> MFTRFVTQPTLLTQTQRALFSALTKKQKMEVTLRTPYKEYLANFDGFSRITAKTNEASLVIQNKTPASLYVLPPGPLKIRFTSEVKNVSGDFLHTGGWVIVHADNTCEI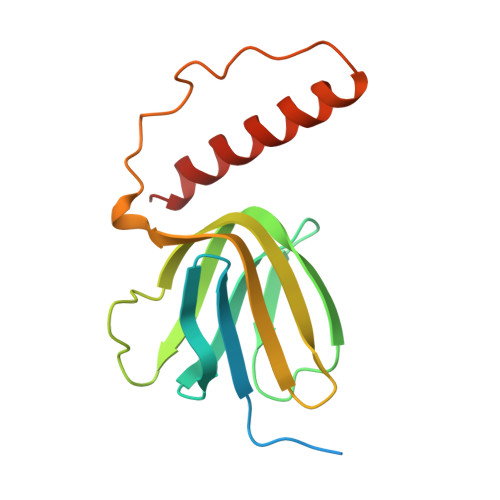NVMDLFDRKEVRADQFEKGNIQDLDTLAGKYAAKSRKSTVRLFTKATTQ> SPPKRLTREAMRNYLKERGDQTVLILHAKVAQKSYGNEKRFFCPPPCVYLMGSGWKKKKEQMERDGCSEQESQPCAFIGIGNSDQEMQQLNLEGKNYCTAKTLYISDSDKRKHFMLSVKMFYGNSDDIGVFLSKRIKVISKPSKKKQSLKNADLCIASGTKVALFNRLRSQTVSTRYLHVEGGNFHASSQQWGAFYIHLLDDDESEGEEFTVRDGYIHYGQTVKLVCSVTGMALPRLIIRKVDKQTALLDADDPVSQLHKCAFYLK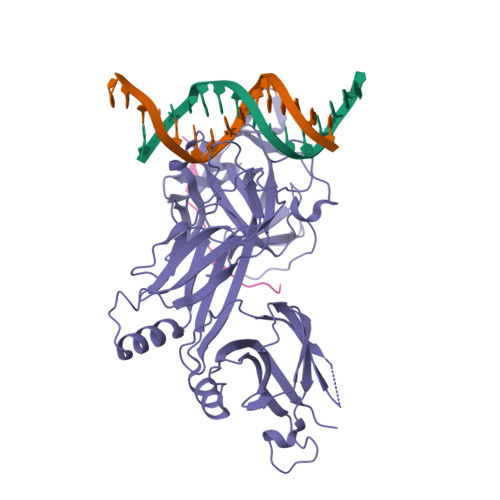DTERMYLCLSQERIIQFQATPCPKEQNKEMINDGASWTIISTDKAEYTFYEGMGPVLAPVTPVPVVESLQLNGGGDVAMLELTGQNFTPNLRVWFGDVEAETMYRCGESMLCVVPDISAFREGWRWVRQPVQVPVTLVRNDGVIYSTSLTFTYTPEP;> ARRKREHSTLWFPEGFSL> TSCNPSDMSHGYVTVKPRVRLHFVELGSGPAVCLCHGFPESWYSWRYQIPALAQAGYRVLAMDMKGYGESSAPPEIEEYCMEVLCKEMVTFLDKLGLSQAVFIGHDWGGMLVWYMALFYPERVRAVASLNTPFIPANPNMSPLESIKANPVFDYQLYFQEPGVAEAELEQNLSRTFKSLFRASDESVLSMHKVCEAGGLFVNSPEEPSLSRMVTEEEIQFYVQQFKKSGF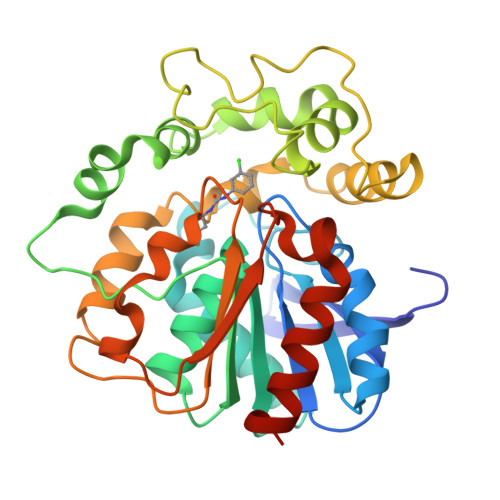RGPLNWYRNMERNWKWACKSLGRKILIPALMVTAEKDFVLVPQMSQHMEDWIPHLKRGHIEDCGHWTQMDKPTEVNQILIKWLDSDARNPPVVSKM> MAADSTITIRGYVRDNGCSVAAESTNFTVDLMENAAKQFNNIGATTPVVPFRILLSPCGNAVSAVKVGFTGVADSHNANLLALENTVSAASGLGIQLLNEQQNQIPLNAPSSAL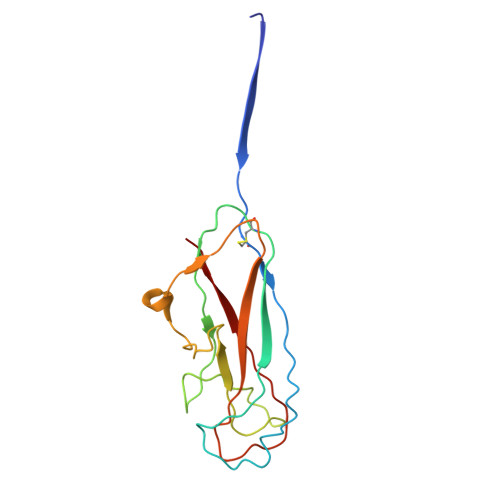SWTTLTPGKPNTLNFYARLMATQVPVTAGHINATATFTLEYQ>[4x]MENLKLDSFLEYKFLSNLDFNPDGSNLAFSLSEADLENNSYKHFIYNLDTKNKEIKKLTHSGKEKNSLWLNNNTILFSADRDKDIEEKKKLGETWTIFYALDIKNGGEAYEYMKLPVNVTEIKIIDENNFILTADFDNNSLNLNDLKGGEREKAIKQIEENKDYEVLDEIPFWSNGNGFRNKKRNRLYHFDKSNNKLTPISDEYTNVESFNIKENKVIFVGRTYKDKQALTAGLYTYDVKSNKLEIIISDNLYDISYANFIEDKIICALSDMKEYGINENHKIYLIDSNKNINLLYENDTWLACTVGSDCRLGGGKSFKVIGNKLYFLSTIADSVHLSSLDTN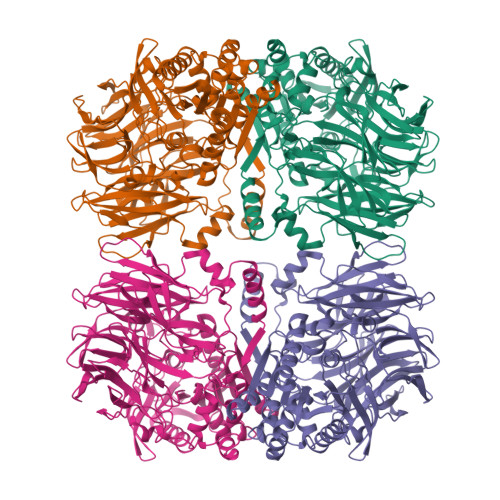GKVEILSSENGSIDFFDIANNEIYYVGMRDYTLQEIYKLENNSSIKLSSFNEEINKKYKISKPEVFDFITNGDTTKGFVIYPIDYDKNKTYPAILDIHGGPKTVYGDVYYHEMQVWANMGYFVIFTNPHGSDGYGNKFADIRGKYGTIDYEDLMNFTDYVLEKYPIDKSRVGVTGGSYGGYMTNWIIGHTDRFKCAASQRSISNWISKFGTTDIGYYFNADQNQATPWINHDKLWWHSPLKYADKAKTPTLFIHSEEDYRCWLAEGLQMFTALKYHGIEARLCMFRGENHELSRSGKPKHRIRRLTEITNWFEKYLK>[2x]SLEGGVVVPVDYHLLMMFTKAEHNAPLQAKARVALSSLLRLAKFEAHEVLNLHFVSEEASREVAKALLRELLPPAAGFKCKVIFHDVAVLTDKLFPVVEAMQKYFSAGSGTYYSDSIFFLSVAMHQIMPKEIPRIIQLDLDLKYKTNIRELFEEFDNFLPGAVIGIAREMQPVYRHTFWQFRHENPKTRVGDPPPEGLPGFNSGVMLLNLEAMRQSPLYSHL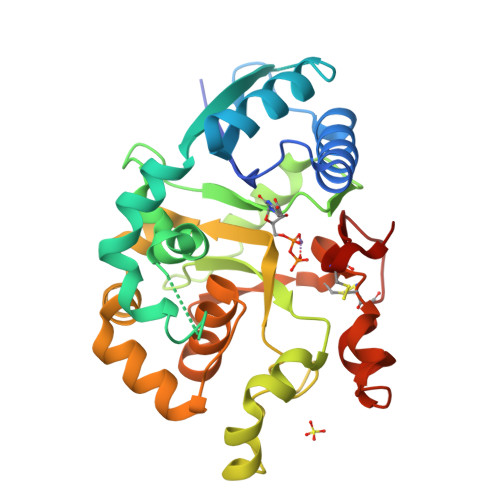LEPSWVQQLADKYHFRGHLGDQDFFTMIGMEHPELFHVLDCTWNRQLCTWWRDHGYSDVFQAYFRCEGHVKIYHGNCNTPIPED> GAQVSTQKTGAHETRLNASGNSIIHYTN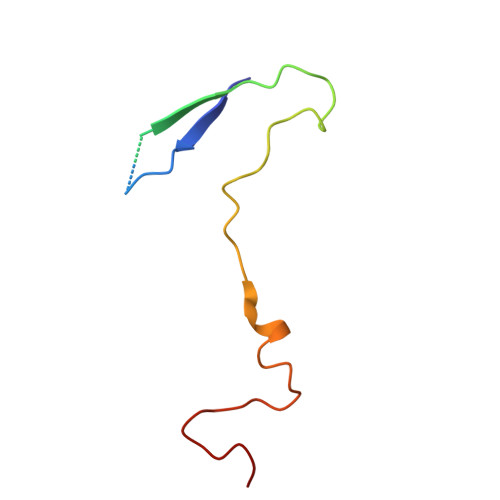INYYKDAASNSANRQDFTQDPGKFTEPVKDIMIKSLPALN> ASLTEIEHLVQSVCKSYRETCQLRLEDLLRQRSNIFSREEVTGYQRKSMWEMWERCAHHLTEAIQYVVEFAKRLSGFMELCQNDQIVLLKAGAMEVVLVRMCRAYNADNRTVFFEGKYGGMELFRALGCSE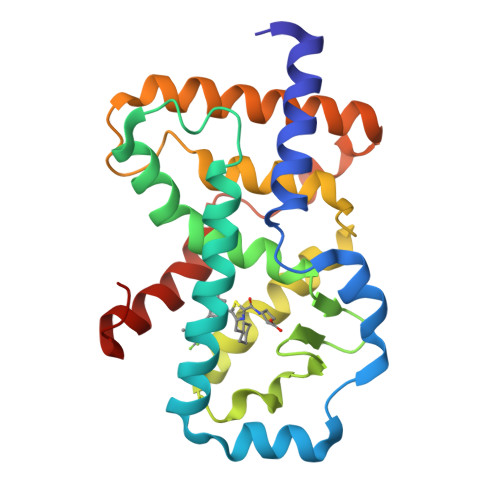LISSIFDFSHSLSALHFSEDEIALYTALVLINAHRPGLQEKRKVEQLQYNLELAFHHHLCKTHRQSILAKLPPKGKLRSLCSQHVERLQIFQHLPA Enteropathogenic *E. coli* (EPEC) O127:H6 encodes an additional, tripartite TA module, *hipBST*, for which the HipT toxin was shown to specifically target tryptophanyl-tRNA synthetase, TrpS. Surprisingly, the function as antitoxin has been taken over by the third protein, HipS, but the molecular details of how activity of HipT is controlled remain poorly understood. Here, we show that HipBST is markedly different from HipBA and that the unique HipS protein, which is homologous to the N-terminal subdomain of HipA, has evolved to function as antitoxin by breaking the kinase active site. We also show how auto-phosphorylation at two conserved sites in the kinase toxin serve to dually regulate binding of HipS and kinase activity.

To understand the molecular basis for the functional and structural differences, we determined the crystal structure of HipBST from enteropathogenic *E. coli* O127:H6 expressed with inactive HipT (D233Q) to 2.9 Å by molecular replacement using HipA_Ec_ as search model ([Fig fig2]). The refined structure (R=19.5% / R_free_=22.8%) has two copies of each of the three proteins in the asymmetric unit and is generally well-defined for HipB and HipT, while HipS appears to be more flexible. Analysis by the protein interaction server, PISA, suggests that the biological assembly is comprised of a dimer of HipBST heterotrimers, which are held together through dimerisation of HipB ([Fig fig2]). In this complex, the two HipB monomers interact strongly (interface area = 1,405 Å^2^) while the interface between HipB and HipT is relatively small (513 Å^2^). The biological relevance of the hetero-hexamer is supported by analytical gel filtration ([Fig figS2]) and small-angle X-ray scattering (SAXS, [Fig figS6]), the latter of which showed a major species with a total mass of 129 ± 8 kDa, in good agreement with the theoretical mass of 125.6 kDa. In the HipBST crystal structures, we find the Gly-rich loop of HipT forms a short α-helix and is in a conformation most similar to the ejected form of the HipA_Ec_ loop despite HipT not being phosphorylated ([Fig fig3]). In this conformation, Ser59, which is known to undergo autophosphorylation in HipT, forms interactions to several active site residues, including Asp210 and the Ser57 auto-phosphorylation site. We conclude that inside the HipBST complex, HipT in its non-phosphorylated state is maintained in an inactive conformation that does not support ATP binding. Near the Gly-rich loop, HipS Glu63 points directly into the HipT active site while Trp65 is wedged into a deep cavity formed by the HipT Gly-rich loop in its outward conformation. We conclude that Trp65 is essential for the ability of HipS to inhibit HipT, presumably either by increasing the affinity of HipS for HipT, or by preventing the Gly-rich loop from adopting the conformation required for ATP binding.

>[2x]ICSGPQNLAQELKAIGDQLQELQKKLIQGPNISQPRPLLTIETPRHLGEQLNARRKELGIDLYTLELQTGISTSTLKRLFKDPEQVKFGSVFAVANVLGVKLCIGE;>HRRVKVLLYGQVVGELSQNDSGFLFQYAHDYHGPAISISLPVAQRQFPSETLHPYFASLAPEGWLRQRYSQIQHRDENDLLGMLIDNGKNLLGAIQILPWEE[2x];>ANCRILLTPLNERDEQRGYSTQGLKRLSGTAKLNPRLGFTRTQFVQELPRQQKGMSISGYQPKLQLVLDEGEFRVVDHQGNFILKPSPADFPGLAENEHATMTLMSRLGFDVPVHGLLSFAPQSEEELEYAFVIRRYDRDNKGLPVHQEQLDGAMQITDKYGKTGNDNEQYVSYETLARFLVAHVNDNIAFKIDLFRRIVYAWLLGNNDMHLRNFGLVYSDGLTPALAPVYQFVSVAPYPEYFYSNYLALPLLTREEGGRELAPGFHSDYGEYIGQDFLLLGESMGLAPRLLEKLFQDIRKENAIVMETYEQSFMTQDHIQAVLQCYRHRLGLLHHHHHH[2x]> GGIQ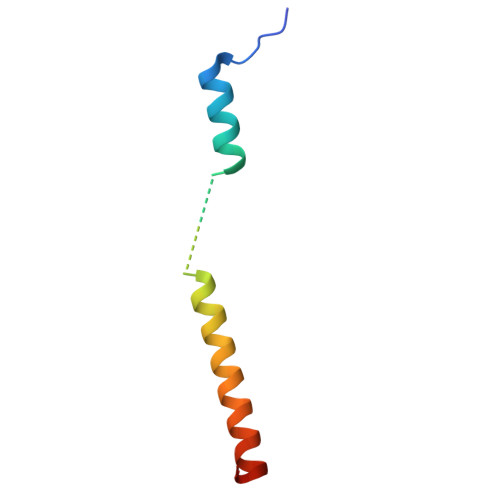RPSLEERLESIISGAALMADSSCTRDDRRERIVAECNAVRQALQDLLSEYMGNAG>PKVNLYATFRDLTGKSQLELPGATVGEVLENLVRAYPALKEELFEGEGLAERVSVFLEGRDVRYLQGLSTPLSPGATLDLFPPVAGGGFERTFGAFPPWLLERYLEEWGGTREGEGVYRL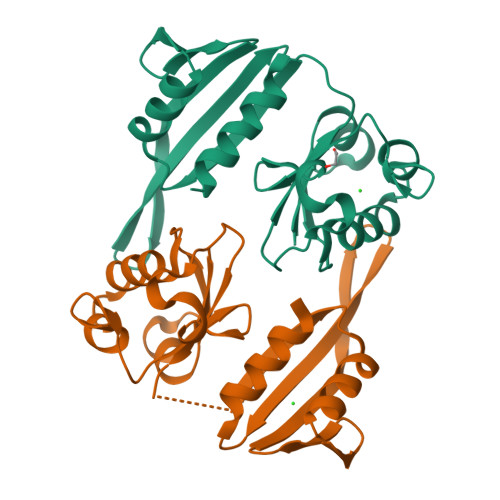PGAVVRFREVEPLKVGSLSIPQLRVEVEGEEAERWFERIAFAASRGGG[4x]SAP05 is an effector from a plant pathogenic phytoplasma that mediates the degradation of host transcription factors, including SPL and GATA family proteins, by hijacking the 26 S plant ubiquitin receptor RPN10 independently of substrate ubiquitination. Specifically, SAP05 folds into a tight globular structure consisting of a parallel five-stranded β-sheet (β1-β5). Although SAP05 carries a single domain, it utilizes two opposing surfaces (hereafter referred to as Lobe1 and Lobe2) to interact simultaneously with TFs and AtRPN10, forming a dumbbell-shaped structure, in which TFs and AtRPN10 have no direct surface contacts. In summary, SAP05 bridges the TFs mainly through electrostatic interactions with a hydrophobic core, whereas the SAP05-AtRPN10 interface comprises predominantly extensive hydrophobic contacts.

In the SAP05-AtRPN10 crystal structure, one asymmetric unit contains two SAP05-AtRPN10 binary complexes with almost identical architecture. Interestingly, the N-terminal loop (L1) of SAP05 becomes a β-strand by packing against its counterpart, forming an antiparallel β-sheet in the crystallographic packing. Appropriately, the α1 and α2 helices of vWA domain, which are not directly involved in the interactions with other subunits of the 19 S regulatory particle, pack against SAP05. In contrast to the acidic Lobe1, the Lobe2 possesses a strong hydrophobic path for AtRPN10 binding, where a cluster of hydrophobic residues including Leu35, Leu73 and Leu69 on the α1-2 helices of AtRPN10 plus Phe49, Phe58, Ile47, Phe61 and Tyr127 on the Lobe2 lining the central interface. While at the edge of α1 helix of vWA domain, the side chains of Gln27 and Glu31 are accommodated by hydrogen bonds with the backbones of Thr48 and Ser50 of SAP05, respectively. Of note, a number of water molecules permeated the Lobe2 and vWA interface, with multiple molecules mediating contacts between SAP05 and AtRPN10. As a result, this binary complex buries a total of 833Å2 of solvent accessible surface area. The results showed that the mutant E31A, L69T or L73D of AtRPN10 was unable to pull down SAP05, suggesting the prominent role of Glu31-mediated hydrogen bonding, and Leu69-, Leu73-mediated hydrophobic interactions in the recognition of SAP05. In light of our SAP05-AtRPN10 structure, we found that residues 38GA39, located on the α1 helix of AtRPN10, do not directly participate in the interaction with SAP05, albeit they are in close proximity to the SAP05 surface. However, the substituted His and Ser residues, especially the bulky His, would induce steric hindrance with the SAP05 surface.

>GAPHEERVGDMRIVNITFSDINSIKNFQPFSQYFDFTLTGPRYNGNIAQFAMIWKIKNPPHNLLGVFFDNNTRDDEDDKYTLEELKQMGNGAKNMYIFWQYEQK[2x];>GMVLEATMICIDNSEWMRNGDYSPSRLQAQTEAVNLLCGAKTQSNPENTVGILTMAGKGVRVLTTPTSDLGKILACMHGLDVGGEINLTAAIQIAQLALKHRQNKNQRQRIIVFAGSPIKYEKKALEIVGKRLKKNSVSLDIVNFGEDDDEEKPQKLEALLTAVNNNDGSHIVHVPSGANALSDVLLSTPVFTG[2x]U6 snRNA is a catalytic RNA responsible for pre-mRNA splicing reactions and undergoes various post-transcriptional modifications during its maturation process. The 3'-oligouridylation of U6 snRNA by the terminal uridylyltransferase, TUT1, provides the Lsm-binding site in U6 snRNA for U4/U6 di-snRNP formation and this ensures pre-mRNA splicing. The oligouridylation of U6 snRNA depends on the internal four-adenosine tract in the 5'-part of the telestem of U6 snRNA, and hTUT1 adds uridines until the internal adenosine tract can form base-pairs with the 3'-oligouridine tract. Together, the recognition of the specific structure and sequence of U6 snRNA by the multi-domain TUT1 protein and the intrinsic sequence and structure of U6 snRNA ensure the oligouridylation of U6 snRNA.

Here, we present the crystal structure of a shortened hTUT1 complexed with a short U6 snRNA, representing the post-uridine addition to the 3'-end of U6 snRNA by hTUT1. Therefore, for a short hTUT1, we designed the hTUT1 lacking the PRR and the KA-1, hereafter termed hTUT1_ΔC. For a shorter U6 snRNA, we designed U6 snRNA lacking the 5'-short stem and the ISL and possessing four 3'-Us (U103-U106), hereafter termed U6_mini. For the crystallization, several cysteine residues in the hTUT1_ΔC were replaced with serine or alanine and one of the catalytic residues, aspartate (Asp218), was replaced with alanine. The crystal belongs to the space group P6522 and contains one hTUT1_ΔC-U6_mini complex in the asymmetric unit cell. Finally, the structure was refined to an Rwork of 30.2% (Rfree = 33.9%) at 3.7 Å resolution. The N-terminal ZF and the RRM constitute a single domain without any linker between them, and the ZF-RRM and the palm of hTUT1_ΔC together clamp the 5'-single stranded region containing the AUA motif of U6_mini. The ZF and the groove loop (amino acid residues 423–427) in the fingers hold the double-stranded telestem from the major and minor grooves of the stem region of U6_mini, respectively, and the 5'-anchor (amino acid residues 357–371) of the palm stacks with the base-pair at the top of the telestem. In the structure of the hTUT1_ΔC-U6_mini complex, the 3'-terminal uridine of U6_mini, corresponding to U106 of U6 snRNA, resides in the incoming UTP-binding site (+1 position) in the catalytic pocket, and the uridine base stacks with the uridine base of U105 (−1 position, 3'-priming position). Thus, the present structure represents the post-U-addition stage.

> MAAVDSDVESLPRGGFRCSLCHVTTANRPSLDAHLGGRKHRHLVELRAARKAQGLRSVFVSGFPRDVDSAQLSEYFLAFGPVASVVMDKDKGVFAIVEMGDVGAREAVLSQSQHSLGGHRLRVRPREQKEFQSPASKSPKGAAPDSHQLAKALAEAADVGAQMIKLVGLRELSEAERQLRSLVVALMQEVFTEFFPGCVVHPFGSSINSFDVHGCDLALFLDLGDLEEPQPVPKLPPASPLLEDREEGDLGKASELAETPKEEKAEGAAMLELVGSILRGCVPGVYRVQTVPSARRPVVKFAHRPSGLHGDVSLSNRLALHNSRFLSLASELDGRVRPLVYTLRAWAQGRGLSGSGPLLSNYALTLLVIYFLQTRDPPVLPTVSQLTQKAGEGEQVEVDGWDCSFPRDASRLEPSINVEPLSSLLAQFFSAVSSWDLRGSLLSLREGQALPVAGGLPSNLWEGLRLGPLNLQDPFDLSHNVAANVTSRVAGRLQNCCRAAANYARSLQYQRRSSRGRDWGLLPLLQPSSLEHHHHHH> MADTQYILPNDIGVSSLDSREAFRLLSPTERLYAYHLSRAAWYGGLAVLLQTSPEAPYIYALLSRLFRAQDPDQLRQHALAEGLTEEEYQAFLVYAAGVYSNMGNYKSFGDTKFVPNLPKEKLERVILGSEAAQQHPEEVRGLWQTCGELMFSLEPRLRHLGLGKEGITTYFSGNCTMEDAKLAQDFLDSQNLSAYNTRLFKEVDGCGKPYYEVRLASVLGSEPSLDSEVTSKLKSYEFRGSPFQVTRGDYAPILQKVVEQLEKAKAYAANSHQGQMLAQYIESFTQGSIEAHKRGSRFWIQDKGPIVESYIGFIESYRDPFGSRGEFEGFVAVVNKAMSAKFERLVASAEQLLKELPWPPTFEKDKFLTPDFTSLDVLTFAGSGIPAGINIPNYDDLRQTEGFKNVSLGNVLAVAYATQREKLTFLEEDDKDLYILWKGPSFDVQVGLHALLGHGSGKLFVQDEKGAFNFDQETVINPETGEQIQSWYRCGETWDSKFSTIASSYEECRAESVGLYLSLHPQVLEIFGFEGADAEDVIYVNWLNMVRAGLLALEFYTPEAFNWRQAHMQARFVILRVLLEAGEGLVTITPTTGSDGRPDARVRLDRSKIRSVGKPALERFLRRLQVLKSTGDVAG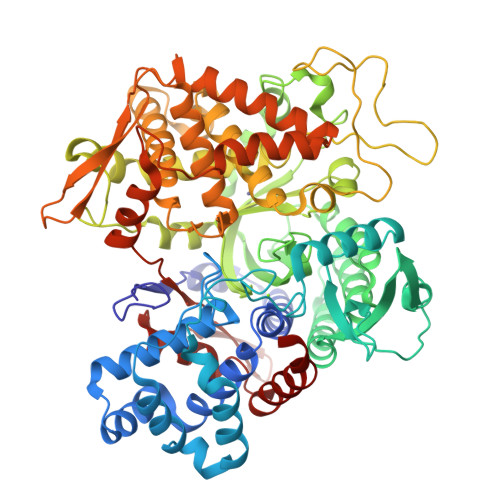GRALYEGYATVTDAPPESFLTLRDTVLLRKESRKLIVQPNTRLEGSDVQLLEYEASAAGLIRSFSERFPEDGPELEEILTQLATADARFW> GKVVLDAVTHPSKIEEAEKLLEEYRERLGGGLEGRVIADPKADPNTGNVHLKTEDGFEVDSTGKDIKTSLDAAL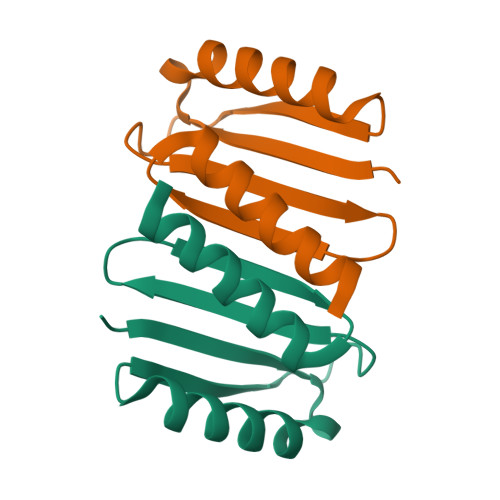AALEWLEHHHHHH>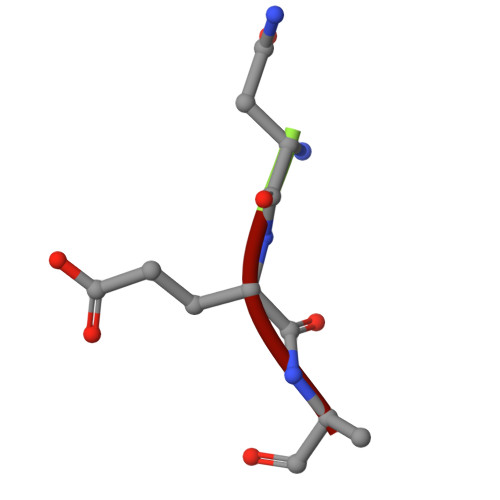 NEA> MEDMILTEEMQKIMNLIQDDENNVFVTGKAGSGKTTFLKYLIEKSGKNCIVAAPTGIAAINAGGVTLHSLFGIPFGPITPYDRLENKFSEYKVELLLKMELLIIDEISMVRPDILDTIDRKLRWVYESDEPFGGVQVIMFGDLFQLPPVTKKQEREILSDFYDGFFFFNALVFKRTGFHIVELTKIFRQTEPEFINVLNNIRNYQVTSDELDLLSELKDRKISSSYDNEYIHICTHKADVEKINADKLGEQEIRNYDIVIKDKFPESSIPCDLHLKLRVGARVMSLVNDSLKGYYNGMLGIVTALEDNVITVRMDNGRTIKFERYTWSNTQYTLKDNEI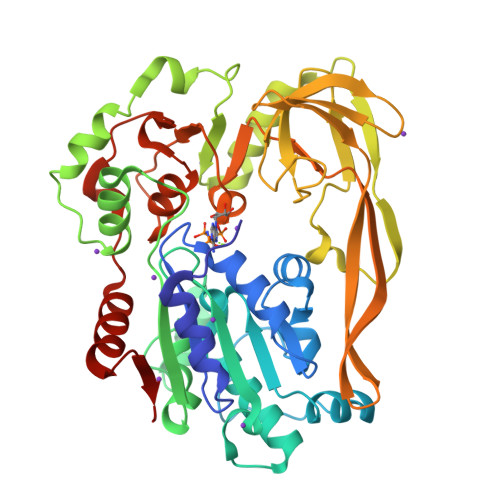VKEEIGSCTQFPLTLAWAITIHKSQGLTFDKIIIHVSHTFCPGQLYVALSRCRTLEGIVSDAFITKQMIIPEYALIDFERAYKSEGNYYGKRLD> G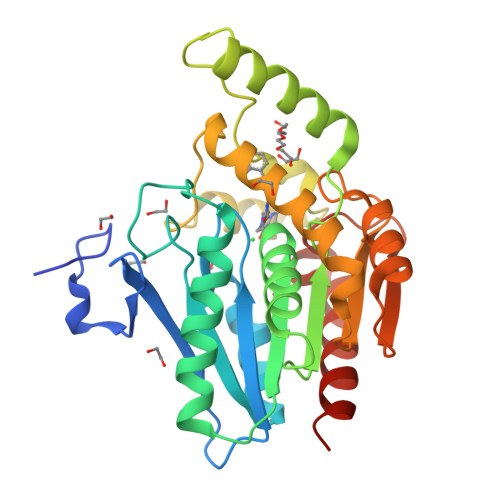SMPEESSPRRTPQSIPYQDLPHLVNADGQYLFCRYWAPTGTPKALIFVSHGAGEHSGRYEELARMLMGLDLLVFAHDHVGHGQSEGERMVVSDFHVFVRDVLQHVDSMQKDYPGLPVFLLGHSMGGAIAILTAAERPGHFAGMVLISPLVLANPESATTFKVLAAKVLNSVLPNLSSGPIDSSVLSRNKTEVDIYNSDPLICRAGLKVCFGIQLLNAVSRVERALPKLTVPFLLLQGSADRLCDSKGAYLLMELAKSQDKTLKIYEGAYHVLHKELPEVTNSVFHEINMWVSQRTATAGTASPP> KPKLLNKFDKTIKAELDAAEKLRKRGKIEEAVNAFKELVRKYPQSPRARYGKAQCEDDLAEKRRSNEVLRGAIETYQEVASLPDVPAD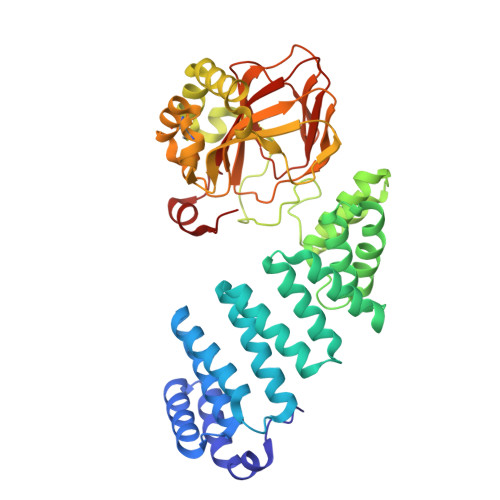LLKLSLKRRSDRQQFLGHMRGSLLTLQRLVQLFPNDTSLKNDLGVGYLLIGDNDNAKKVYEEVLSVTPNDGFAKVHYGFILKAQNKIAESIPYLKEGIESGDPGTDDGRFYFHLGDAMQRVGNKEAYKWYELGHKRGHFASVWQRSLYNVNGLKAQPWWTPKETGYTELVKSLERNWKLIRDEGLAVMDKAKGLFLPEDENLREKGDWSQFTLWQQGRRNENACKGAPKTCTLLEKFPETTGCRRGQIKYSIMHPGTHVWPATGPTNCRLRMHLGLVIPKEGCKIRCANETKTWEEGKVLIFDDSFEHEVWQDASSFRLIFIVDVWHPELTPQQRRSLPAI>[2x]MSLNYIEDIKNYIPFNEQEERDKELFLRCLNDFHDILTRDNTIAHLTSSAFAVNKERNKFLMIHHNIYNSWAWTGGHSDNEKDQLKVAIKELKEETGVKNPTPLLDK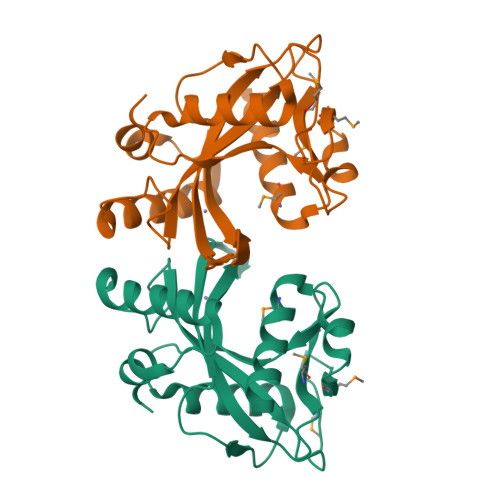AFALDVLTVNGHIKRGKYVSSHLHLNLTYLIECSEDETLMLKEDENSGVMWIPFNEISKYCSEPHMIPIYEKLINKLKTQSKEGHHHHHH(2S,3R)-2-azanyl-N-[5-(7-bromanyl-6-chloranyl-4-oxidanylidene-quinazolin-3-yl)pentyl]-3-oxidanyl-N-[[3-(1-oxidanylidene-2,3-dihydroisoindol-5-yl)phenyl]methyl]butanamide 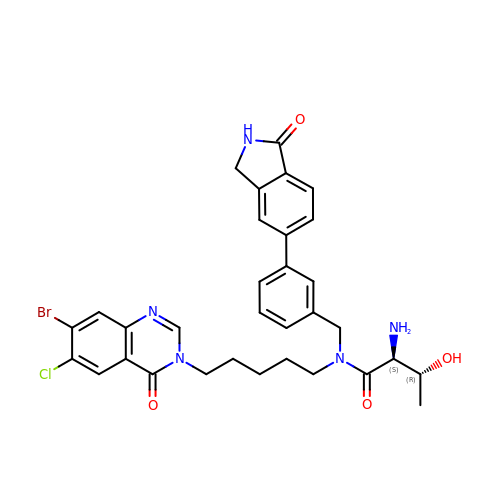| C32 H33 Br Cl N5 O4 | BLRJMFLSHHBCFQ-XBBWARJSSA-N> MKTMRKQIYKKAYWLLLPFLPLALANTFLVKEDSKNVTAYTPFATPITDSKSDLVSLAQLDSSYQIADQTIHNTNLFVLFKSRDVKVKYESSGSNNISFDSTSQGEKPSYVVEFTNSTNIGIKWTMVKKYQLDVPNVSSDMNQVLKNLILEQPLTKYTLNSSLAKEKGKTQREVHLGSGQANQWTSQRNQHDLNNNPSPNASTGFKLTTGNAYRKLSESWPIYEPIDGTKQGKGKDSSGWSSTEENEAKNDAPSVSGGGSSSGTFNKYLNTKQALESIGILFDDQTPRNVITQLYYASTSKLAVTNNHIVVMGNSFLPSMWYWVVERSAQENASNKPTWFANTNLDWGEDKQKQFVENQLGYKETTSTNSHNFHSKSFTQPAYLISGIDSVNDQIIFSGFKAGSVGYDSSSSSSSSSSSSTKDQALAWSTTTSLDSKTGYKDLVTNDTGLNGPINGSFSIQDTFSFVVPYSGNHTNNGTTGPIKTAYPVKKDQKSTVKINSLINATPLNSYGDEGIGVFDALGLNYNFKSNQERLPSRTDQIFVYGIVSPNELRSAKSSADSTGSDTKVNWSNTQSRYLPVPYNYSEGIIDADGFKRPENRGASVTTFSGLKSIAPDGFANSIANFSVGLKAGIDPNPVMSGKKANYGAVVLTRGGVVRLNFNPGNDSLLSTTDNNIAPISFSFTPFTAAESAVDLTTFKEVTYNQESGLWSYIFDSSLKPSHDGKQTPVTDNMGFSVITVSRTGIELNQDQATTTLDVAPSALAVQSGIQSTTQTLTGVLPLSEEFSAVIAKDSDQNKIDIYKNNNGLFEIDTQLSNSVATNNGGLAPSYTENRVDAWGKVEFADNSVLQARNLVDKTVDEIINTPEILNSFFRFTPAFEDQKATLVATKQSDTSLSVSPRIQFLDGNFYDLNSTIAGVPLNIGFPSRVFAGFAALPAWVIPVSVGSSVGILFILLVLGLGIGIPMYRVRKLQDASFVNVFKKVDTLTTAVGSVYKKIITQTGVVKKAPSALKAANPSVKKPAAFLK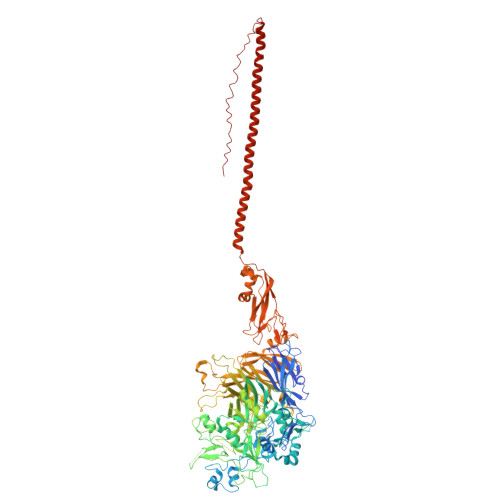PPVQPPSKPEGEQKAVEVKSEETKS2-amino-5-{2-[(1S)-1-cyclopropylethyl]-7-methyl-1-oxo-2,3-dihydro-1H-isoindol-5-yl}-N-(trans-3-hydroxycyclobutyl)pyrazolo[1,5-a]pyrimidine-3-carboxamide 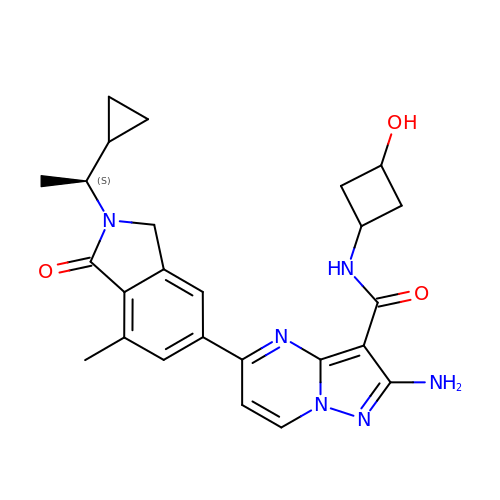| C25 H28 N6 O3 | DKTOKFSQYVFDRK-KKXDTOCCSA-N>GKNPVESVSVEFEAKSARDGAWYDVAAFLSHRLFESGDPEVRVRFSGFGAEEDEWINVRKCVRQRSLPCEATECVAVLPGDLILCFQEGKDQAL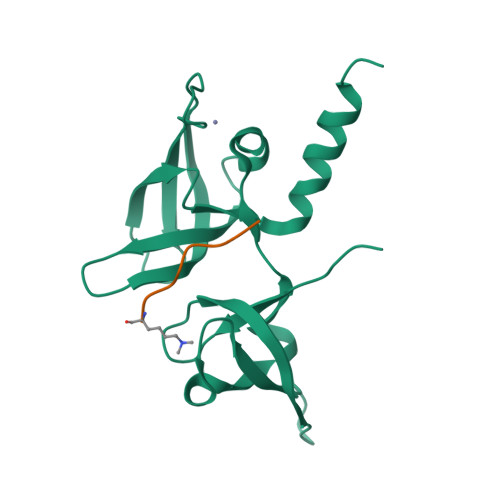YYDAHVLDAQRRRHDVGGCRCRFLVRYDHDSSEEIVPLRKVCRRPETDYRLQILHAARAAATN[2x];>[2x]ARTKQTARKS> GSEGHRTLASTPALWASIPCPRSELRLDLVLPSGQSFRWREQSPAHWSGVLADQVWTLTQTEEQLHCTVYRGDKSQASRPTPDELEAVRKYFQLDVTLAQLYHHWGSVDSHFQEVAQKFQGVRLLRQDPIECLFSFICSSNNNIARITGMVERLCQAFGPRLIQLDDVTYHGFPSLQALAGPEVEAHLRKLGLGYRARYVSASARAILEEQGGLAWLQQLRESSYEEAHKALCILPGVGTQVADCICLMA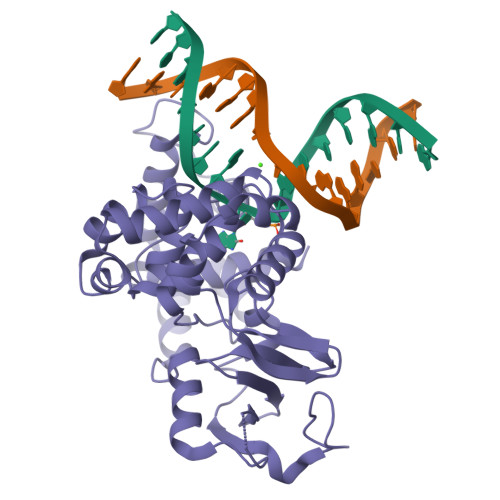LDKPQAVPVDVHMWHIAQRDYSWHPTTSQAKGPSPQTNKELGNFFRSLWGPYAGWAQAVLFSADLRQ>[2x]QGPMESRRESINPWILTGFTDAEGSFMLRIRNTNNRSVGYYTSLVFEITLHNKDKSILENIQSTWKVGTINNRGDGTARLSVTRFEDLKVIIDHFEKYPLITQKLGDYKLFKQAFSVMENKEHLKENGIKELVRIKAKMNWGLNDELKKAFPE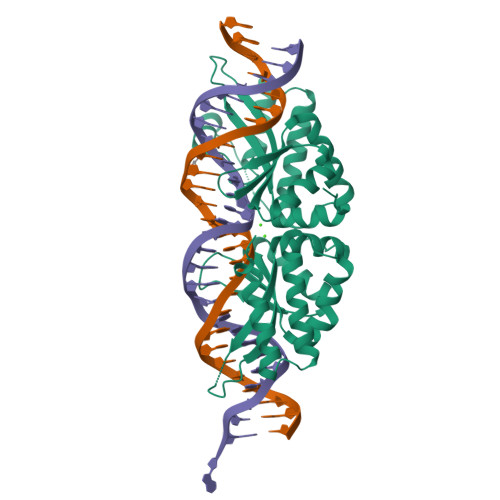NISKERPLINKNIPNLKWLAGFTSGEGTFYVHLAKSEASGKVYVRLRFIIGQHIRDKNLMNSLITYLGCGTIQEKNRSKGSMLHFIVTKFSDINDKIIPVFQENTLIGVKLEDFEDWCKVAKLIEEKKHLTESGLDEIKKIKLNMNKGRVF>ETGIGQRIVCLVLDKSGSMATGNRLNRLNQAGQLFLLQTVELGSWVGMVTFDSAAHVQSELIQINSGSDRDTLAKRLPAAASGGTSICSGLRSAFTVIRKKYPTDGSEIVLLTDGEDNTISGCFNEVKQSGAIIHTVALGPSAAQELEELSKMTGGLQTYASDQVQNNGLIDAFGALSGTK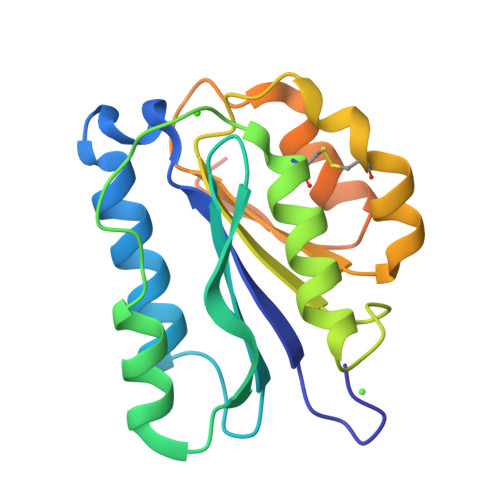HHHHHH[2x]>[2x]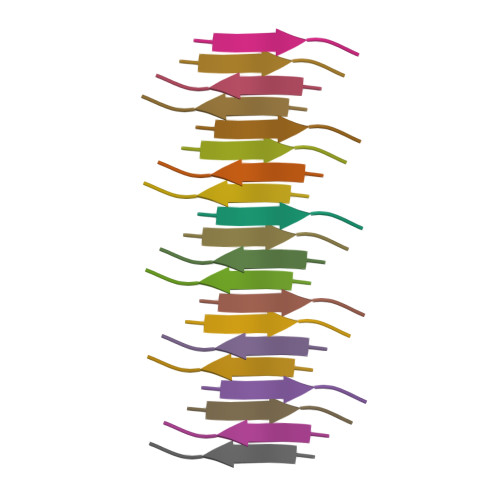AADTWE> MANVWGVRLADSLSSPTIETRTRQYTLHDLCSDLDANPGREPWKPLRNQRTNNIVAVQLFRPLQGLVLDTQLYGFPGAFDDWERFMREKLRVLKYEVLRIYPISNYSNEHVNVFVANALVGAFLSNQAFYDLLPLLIINDTMIGDLLGTGASLSQFFQSHGDVLEVAAGRKYLQMENYSNDDDDPPLFAKDLSDYAKAFYSDTYEVLDRFFWTHDSSAGVLVHYDKPTNGHHYLLGTLTQMVSAPPYIINATDAMLLESCLEQFSANVRARPAQPVTRLDQCYHLRWGAQYVGEDSLTYRLGVLSLLATNGYQLARPIPRQLTNRWLSSFVSQIMSDGVNETPLWPQERYVQIAYDSPSVVDGATQYGYVRKNQLRLGMRISALQSLSDTPSPVQWLPQYTIDQAAMDEGDLMVSRLTQLPLRPDYGNIWVGDALSYYVDYNRSHRVVLSSELPQLPDTYFDGDEQYGRSLFSLARKIGDRSLVKDTAVLKHAYQAIDPNTGKEYLRSRQSVAYFGASAGHSGADQPLVIEPWIQGKISGVPPPSSVRQFGYDVARGAIVDLARPFPSGDYQFVYSDVDQVVDGHDDLSISSGLVESLLSSCMHATAPGGSFVVKINFPTRPVWHYIEQKILPNITSYMLIKPFVTNNVELFFVAFGVHQHSSLTWTSGVYFFLVDHFYRYETLSTISRQLPSFGYVDDGSSVTGIETISIENPGFSNMTQAARIGISGLCANVGNARKS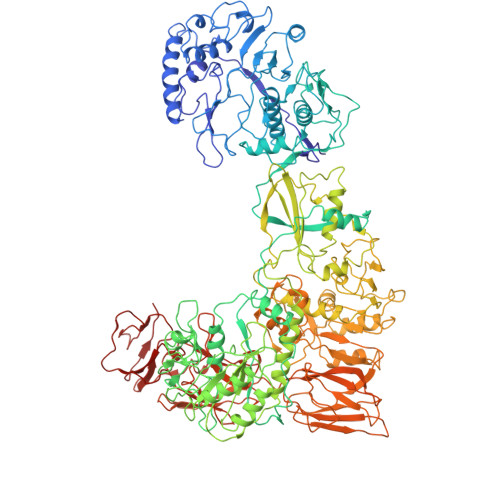IAIYESHGARVLTITSRRSPASARRKSRLRYLPLIDPRSLEVQARTILPADPVLFENVSGASPHVCLTMMYNFEVSSAVYDGDVVLDLGTGPEAKILELIPATSPVTCVDIRPTAQPSGCWNVRTTFLELDYLSDGWITGVRGDIVTCMLSLGAAAAGKSMTFDAAFQQLIKVLSKSTANVVLVQVNCPTDVVRSIKGYLEIDSTNKRYRFPKFGRDEPYSDMDALEKICRTAWPNCSITWVPLSYDLRWTRLALLESTTLSSASIRIAELMYKYMPIMRIDIHGLPMEKRGNFIVGQNCSLVIPGFNAQDVFNCYFNSALAFSTEDVNAAMIPQVSAQFDATKGEWTLDMVFSDAGIYTMQALVGSNANPVSLGSFVVDSPDVDITDAWPAQLDFTIAGTDVDITVNPYYRLMTFVRIDGQWQIANPDKFQFFSSASGTLVMNVKLDIADKYLLYYIRDVQSRDVGFYIQHPLQLLNTITLPTNEDLFLSAPDMREWAVKESGNTICILNSQGFVLPQDWDVLTDTISWSPSIPTYIVPPGDYTLTPL>APQQINDIVHRTITPLIEQQKIPGMAVAVIYQGKPYYFTWGYADIAKKQPVTQQTLFELGSVSKTFTGVLGGDAIARGEIKLSDPTTKYWPELTAKQWNGITLLHLATYTAGGLPLQVPDEVKSSSDLLRFYQNWQPAWAPGTQRLYANSSIGLFGALAVKPSGLSFEQAMQTRVFQPLKLNHTWINVPPAEEKNYAWGYREGKAVHAAAVSPGALDAEAYGVKSTIEDMARWVQSNLKPLDINEKTLQQGIQLAQSRYWQTGDMYQGLGWEMLDWPVNPDSIINGSDNKIALAARPV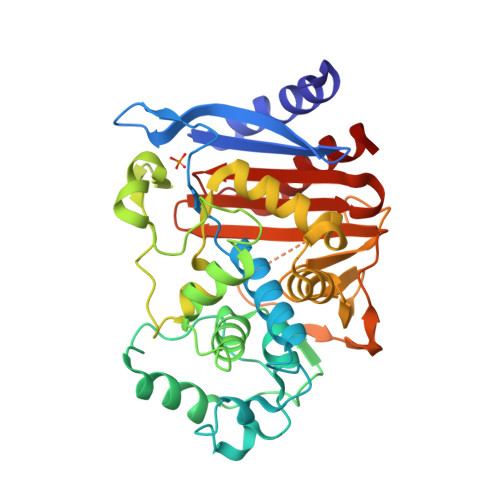KAITPPTPAVRASWVHKTGATGGFGSYVAFIPEKELGIVMLANKNYPNPARVDAAWQILNALQ[2x]2-[(R)-(2-chlorophenyl){2-[(2S)-1-methylpyrrolidin-2-yl]ethoxy}methyl]thieno[3,2-b]pyridine-7-carboxylic acid | C22 H23 Cl N2 O3 S | 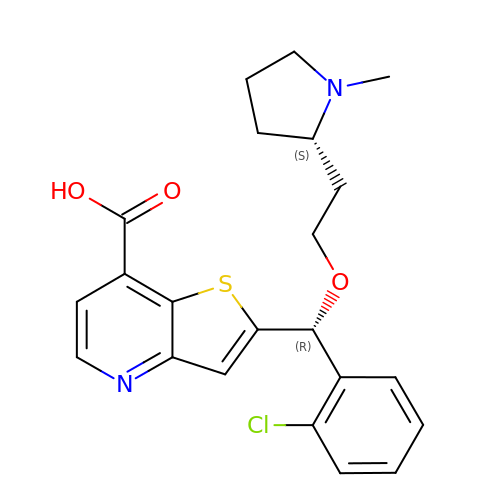CKHGFLIUOABPPV-VBKZILBWSA-N> SVAEINAQYYQQESA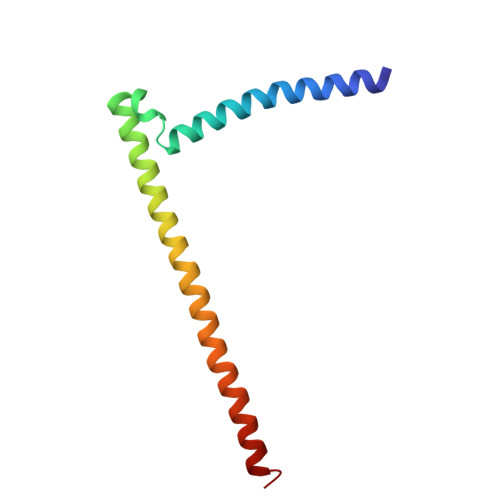KLRQQIISIQNSNRQLMGETIGSMSPKELRNLEGRLERSITRIRSKKNELLFSEIDYMQKREVDLHNDNQILRAKIAENRN Particularly striking is the much larger size (~260 amino acids) of their single capsid or core proteins (CPs) which in mammalian HBVs comprise only ~180 aa. DHBV CP (DHBc) expressed in E. coli self-assembles into CLPs which package bacterial RNA. In line with earlier data the major type of DHBc CLP conformed to the clustered-dimer T = 4 architecture known from HBc. Confirming selective aspects of evolutionary conservation between avi- and orthohepadnaviruses, the new data also reveal unique structural modules, including a direct contribution of the very C-terminal residues to the capsid shell and a centrally inserted extension of ~45 aa that behaves like an independent folding entity.

The 3D-map of the CLPs had a resolution of 3.7 Å, but more importantly, the extension domains were clearly visible at the same threshold as the core of the spikes, indicating that during long-term storage most extension domains had become folded. Local refinement of the orientations of these particles further improved the overall resolution of the asymmetric unit to a nominal resolution of 3 Å with the extension domains still less well resolved than the rest of the asymmetric unit. The core of the spikes was formed by four helices, with each DHBc monomer contributing an ascending helix (α3; residues 44–78, 35 aa) and a descending helix (α4; residues 120–157, 38 aa). The ascending helix α3 was kinked in the center between F60 and W61 and tilted away from the dimer axis in the upper part of the spike. Moreover, DHBc helices α3 and α4 were connected through a 41 aa long extension domain (residues 79–119) whereas in HBc this connection is just a short loop of 3–4 aa. The extension with two short helical segments (αe1: 92–99; αe2: 103–117), was positioned at the side of the spike close to α4 of the same subunit and in contact with α3 of the other subunit. As independently confirmed below, the packing of the extension domain to the flank of the spike was stabilized by a salt bridge between R124 in α4 of the core spike and E109 in αe2 of the extension domain. Analysis with Intersurf showed that the extension domain increased the inter-dimer surface area from ~1,900 Å² to ~3,400 Å², highlighting its important contribution to the intra-dimer contact. In DHBc the seven N-terminal residues pointed towards the lumen of the capsid, without contributing to the intra-dimer contact. The pockets at the base of the spikes close to the N-termini of chains A and D contained density that was not accounted for by the so far described model (f magenta). This density resembled a short peptide and was modelled with the 13 very C-terminal residues 250–262.

>[6x]MDINASRALANVYDLPDDFFPKIDDLVRDAKDALEPYWKSDSIKKHVLIATHFVDLIEDFWQTTQGMHEIAESLRAVIPPTTTPVPPGYLIQHEEAEEIPLGDLFKHQEERIVSFQPDYPITARIHAHLKAYAKINEESLDRARRLLWWHYNCLLWGEAQVTNYISRLRTWLSTPEKYRGRDAPTIEAITRPIQVAQGGRKTTTGTRKPRGLEPRRRKVKTTVVYGRRRSKSRERRAPTPQRAGSPLPRSSSSHHRSPSPRK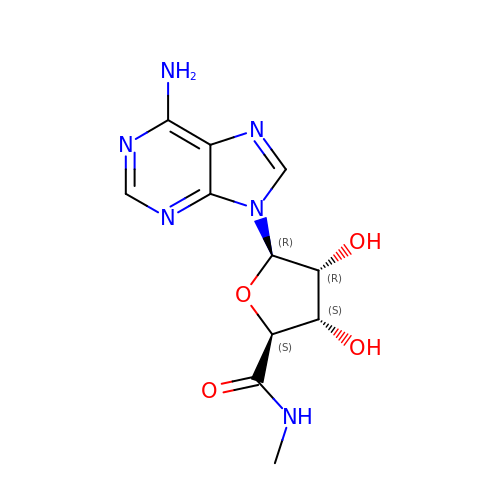(2~{S},3~{S},4~{R},5~{R})-5-(6-aminopurin-9-yl)-~{N}-methyl-3,4-bis(oxidanyl)oxolane-2-carboxamide | C11 H14 N6 O4 | PLYRYAHDNXANEG-QMWPFBOUSA-N>INTITYDAGNTTINKYATFMESLRNEAKDPSLQCYGIPMLPNNSSTIKYLLVKLQGASQKTITLMLRRNNLYVMGYSDPFNGNCRYHIFNDITGTERTNVENTLCSSSS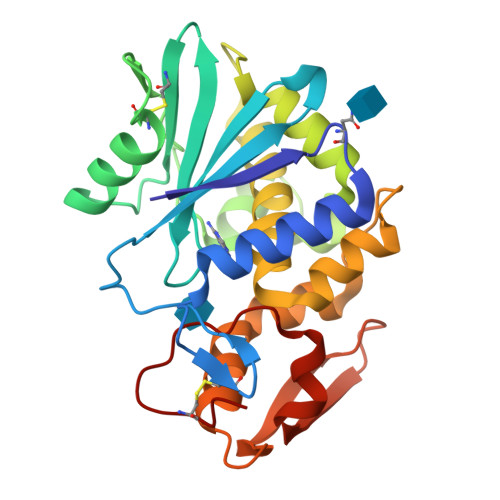SRDAKPINYNSLYSTLEKKAEVNSRSQVQLGIQILSSDIGKISGQSSFTDKTEAKFLLVAIQMVSEAARFKYIENQVKTNFNRDFSPNDKILDLEENWGKISTAIHDATNGALPKPLELKNADGTKWIVLRVDEIKPDMGLLNYVNGTCQTT[2x]>[12x]MSLTLLKGRRKVDTIKVGILGYGLSGSVFHGPLLDVLDEYQISKIMTSRTEEVKRDFPD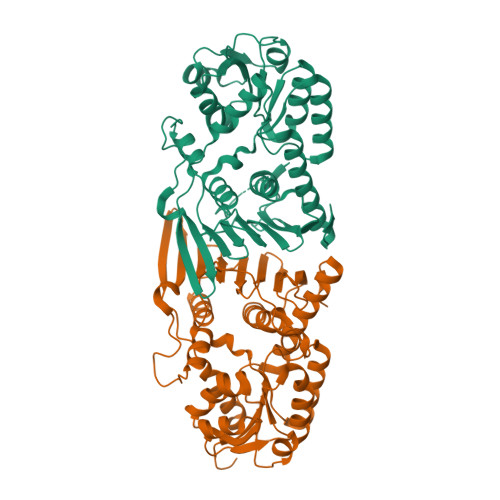AEVVHELEEITNDPAIELVIVTTPSGLHYEHTMACIQAGKHVVMEKPMTATAEEGETLKRAADEKGVLLSVYHNRRWDNDFLTIKKLISEGSLEDINTYQVSYNRYRPEVQARWREKEGTATGTLYDLGSHIIDQTLHLFGMPKAVTANVMAQRENAETVDYFHLTLDYGKLQAILYGGSIVPANGPRYQIHGKDSSFIKYGIDGQEDALRAGRKPEDDSWGADVPEFYGKLTTIRGSDKKTETIPSVNGSYLTYYRKIAESIREGAALPVTAEEGINVIRIIEAAMESSKEKRTIMLEHEGHHHHHH>[2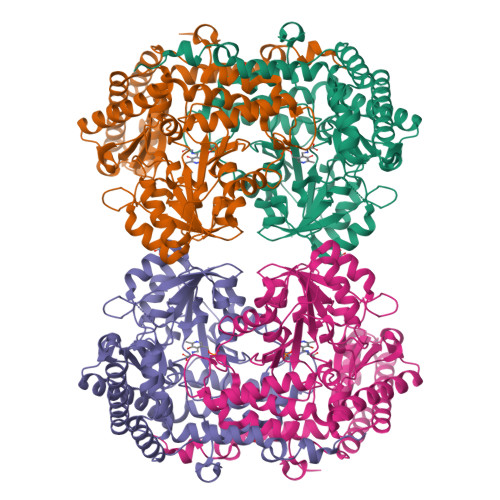x]SHMDPVSVWGNTPLATVDPEIHDLIEKEKRRQCRGIELIASENFTSFAVIEALGSALTNKYSEGMPGNRYYGGNEYIDQIENLCRSRALQAFHLDAQSWGVNVQPYSGSPANFAAYTAVLNPHDRIMGLDLPSGGHLTHGYYTSGGKKISATSIYFESLPYKVNSTTGYIDYDRLEEKALDFRPKLIICGGSAYPRDWDYKRFREVADKCGALLLCDMAHTSGLVAAQEVNSPFEYCDIVTTTTHKSLRGPRAGMIFYRKGPKPPKKGQPENAVYDFEDKINFAVFPSLQGGPHNHQIGALAVALKQAASPGFKAYAKQVKANAVALGKYLMGKGYSLVTGGTENHLVLWDLRPLGLTGNKVEKLCDLCNITVNKNAVFGDSSALAPGGVRIGAPAMTSRGLVEKDFEQIGEFLHRAVTLTLEIQKEHGKLLKDFNKGLVNNKAIEDLKADVEKFSALFDMPGFLVSEMKYKD The evolutionarily related deubiquitinating enzymes (DUBs) USP25 and USP28 comprise an identical overall domain architecture but are functionally non-redundant: USP28 stabilizes c-MYC and other nuclear proteins, and USP25 regulates inflammatory TRAF signaling. USP25 and USP28 share an identical domain structure and highly homologous catalytic domains. USP catalytic domains are usually around 350 amino acids (aa) in length; however, in USP25/28, the catalytic domains span ∼550 aa due to a large, conserved insertion of unknown function at a common insertion point between USP boxes 4 and 5 (Ye et al., 2009). Active enzymes form distinctively shaped dimers, with a dimerizing insertion spatially separating independently active catalytic domains.

A C-terminal region comprising ∼340 aa of unknown structure and function, yet with high conservation, is shared by USP25 and USP28. We embarked on structural studies for this domain, excluding a C-terminal peptide in USP25 (aa 1,049–1,055) that facilitates an interaction with tankyrases to mediate their stabilization (Xu et al., 2017). A 1.7-Å crystal structure of USP25 (748–1,048) was solved by ab initio molecular replacement (Bibby et al., 2012) and revealed an α-helical domain without any similarity to previously reported structures in the protein data bank according to DALI. C-terminally extended USP25 (aa 157–1,055) was exclusively tetrameric, indicating that the C-terminal domain does not affect oligomeric behavior per se, as also found for USP28. In full-length enzymes, a C-terminal domain with a previously unknown fold has no impact on oligomerization, but N-terminal regions affect the dimer-tetramer equilibrium in vitro.

> GPDFSKHLKEETIQIITKASHEHEDKSPETVLQSAIKLEYARLVKLAQEDTPPETDYRLHHVVVYFIQNQAPKKIIEKTLLEQFGDRNLSFDERCHNIMKVAQAKLEMIKPEEVNLEEYEEWHQDYRKFRETTMYLIIGLENFQRESYIDSLLFLICAYQNNKELLSKGLYRGHDEELISHYRRECLLKLNEQAAELFESGEDREVNNGLIIMNEFIVPFLPLLLVDEMEEKDILAVEDMRNRWCSYLGQEMEPHLQEKLTDFLPKLLDCSMEIKSFHEPPKLPSYSTHELCERFARIMLSLS>[8x]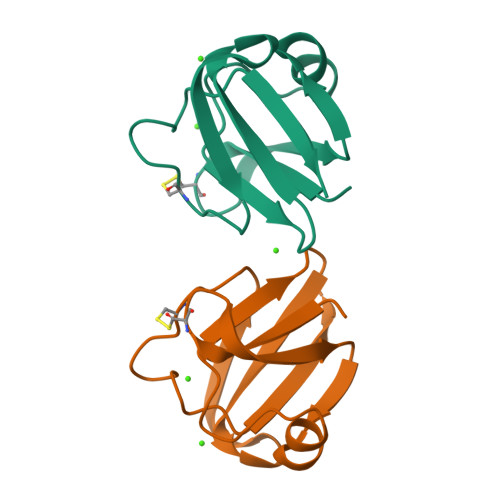DVITVYKDCNYTGFSGGLTIGDYNLARLNSLGVLNDDISSLRITQGYQAILYQDDNFGGASTVINSDNSCLNTTWNDKVSSIRVIANGTT> AEETSFVFSKFKPLEPNLILQGDALVTVAGVLQLTNVDSNGVPEPSSLGRATYSAPINIWDSATGLVASFATSFRFTIYAPNIATIADGLAFFLAPVASAPDSGGGFLGLF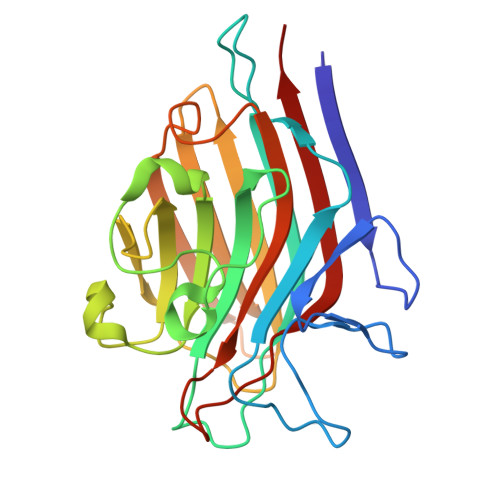DSAVGDTTYQTVAVEFDTYENTVFTDPPYTHIGFDVNSISSIKTVKWSLANGEAAKVLITYNSAVKLLVASLVYPSSKTSFILADIVDLSSVLPEWVRVGFSAATGASKGYIETHDVFSWSFASKLAG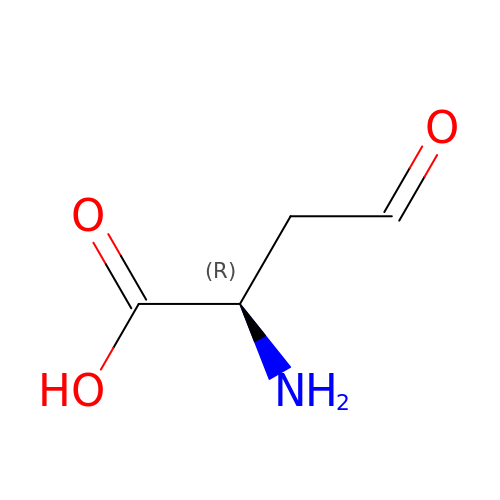(2R)-2-AMINO-4-OXOBUTANOIC ACID | C4 H7 N O3 | HOSWPDPVFBCLSY-GSVOUGTGSA-N> MARRKCRNRFVKKNGQCNVEFTNMDDKPQRYIADMFTTCVDIRWRYMLLLFSLAFLVSWLLFGLIFWLIALIHGDLENPGGDDTFKPCVLQVNGFVAAFLFSIETQTTIGYGFRCVTEECPLAVFMVVVQSIVGCIIDSFMIGAIMAKMARPKKRAQTLLFSHNAVVAMRDGKLCLMWRVGNLRKSHIVEAHVRAQLIKPRITEEGEYIPLDQIDIDVGFDKGLDRIFLVSPITILHEINEDSPLFGISRQDLETDDFEIVVILEGMVEATAMTTQARSSYLASE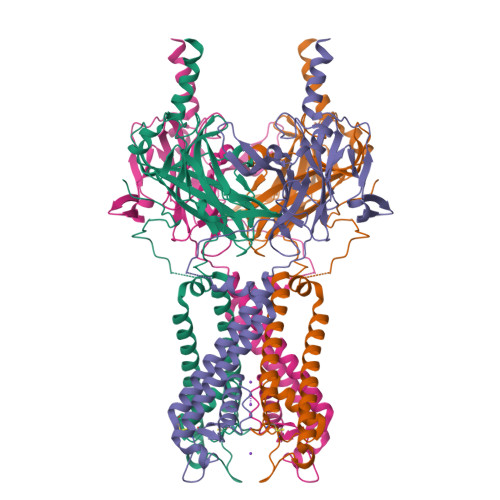ILWGHRFEPVLFEEKNQYKVDYSHFHKTYEVPSTPRCSAKDLVENKFLLSNSLEVLFQ> 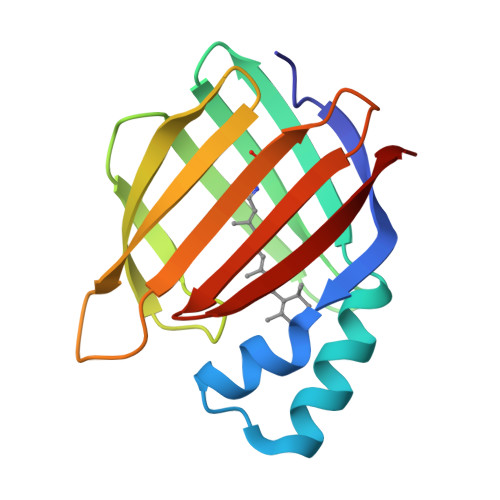PNFSGNWKIIRSENFEELLKVLGVNVMLRKIAVAAASKYAVEIKQEGDTFYIKVSTTVYTTEINFKVGEEFEEQTVDGRPCKSLVKWESENKMVCEQKLLKGEGPKTSWTKELTNDGELIETMTADDVVCTQVFVRE(2-nitro-4-{[(3S)-1-{[4-(trifluoromethyl)phenyl]methyl}pyrrolidin-3-yl]amino}phenyl)methanol 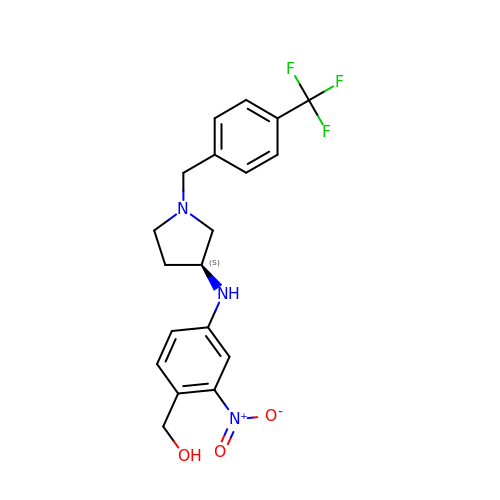| C19 H20 F3 N3 O3 | BDIGVJQSNTVCKR-KRWDZBQOSA-N> HMPSFDFDIPRRSPQEIAKGMVAIPGGTFRMGGEDPDAFPEDGEGPVRTVRLSPFLIDRYAVSNRQFAAFVKATGYVTDAERYGWSFVFHAHVAPGTPVMDAVVPEAPWWVAVPGAYWKAPEGPGSSITDRPNHPVVHVSWNDAVAYATWAGKRLPTEAEWEMAARGGLDQARYPWGNELTPRGRHRCNIWQGTFPVHDTGEDGYTGTAPVNAFAPNGYGLYNVAGNVWEWCADWWSADWHATESPATRIDPRGPETGT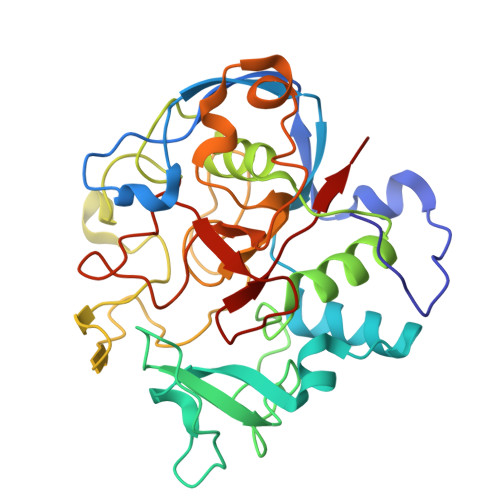ARVTKGGSFLCHESYCNRYRVAARTCNTPDSSAAHTGFRCAADP> QASDVSSNISSLTVSPTQINDGGKTTVRFEFDEHAQNIKAGDTITVNWQNSGTVRGTGYTKTIKLEVQGKYVGDLVVTQDKAVVTFNDSITGLQNITGWGEFEI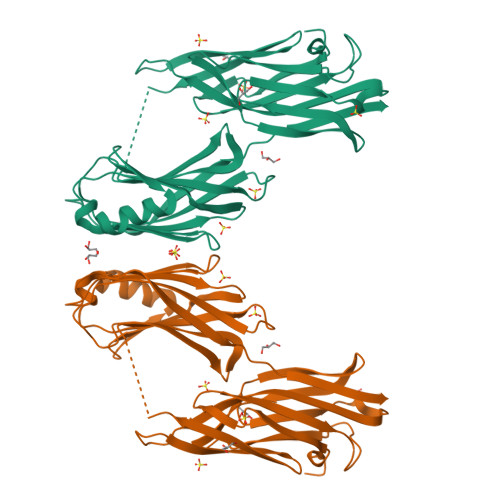EGRNFTDTTTGNTGSFQVTSGGKTAEVTVVKSASGTTGVFYYKTGDMQTDDTNHVRWFLNINNENAYVDSDIRIEDDIQSGQTLDIDSFDITVNGSESYHGQEGINQLAQRYGATISADPASGHISVYIPQGYASLNRFSIMYLTKVDNPDQKTFENNSKAWYKENGKDAVDGKEFNHSVANVNAAGGVDGRLQASSVDKLAAALEHHHHHHHH> KVYYLPVTLTQFQKDLSEILISLHAKSFKASIIGEPQADAVNKPSGLPAGPETHPYP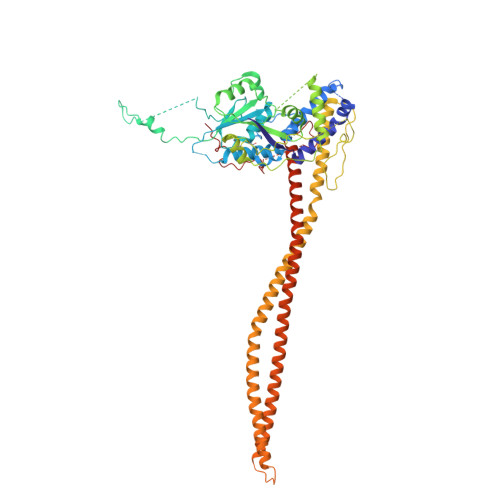TLSQRQLTYIFDSNIRAIANHPSLLVDHYMPRQLLRMEPTESSIAGSHKFQVLNQLINSICFRDREGSPNEVIKCAIIAHSIKELDLLEGLILGKKFRTKRLSGTSLYNEKHKFPNLPTVDSTINKDGTPNSVSSTSSNSNSTSYTGYSKDDYDYSVKRNLKKRKINTDDWLFLATTKHLKHDQYLLANYDIDMIISFDPMLEVELPALQVLRNNANKDIPIIKLLVQNSPDHYLLDSEIKNSSVKSSHLSNNGHVDDSQEYEEIKSSLLYFLQARNAPVNNCEIDYIKLVKCCLEGKDCNNILPVLDLITLDEASKDSSDSGFWQPQLTKLQYSSTELPLWDGPLDIKTYQTELMHRAVIRLRDIQDEYAKGTVPLYEKRLNETQRQNQLDEIKNSVGLTFKKKQEVEKSINDSEKRLKHAMTESTKLQNKINHLLKNRQELENFNKLPSNTISSENHLEEGSALADKLKEYIDKNATLFNKLKELQQANAEKSKLNDELRSKYQIESSKAAESAQTLKILQESMKSLENEVNGPLTKFSTESLKKELERLQNDFQSLKARNKFLKNYITL> MSKGTTCQKAIVNWEAANPGKNPSEAEEIKLIFQIPPIEKMDGPVLNTLTKCKKLSLSSNSIDKMISLNMLRNLEILSLSRNVIKKISGLEDIGGTLRQLWLSYNFIEKLDGLNNCSVLQTLYIGNNRIKNWEELDKLKDLPELENVLFYGNPI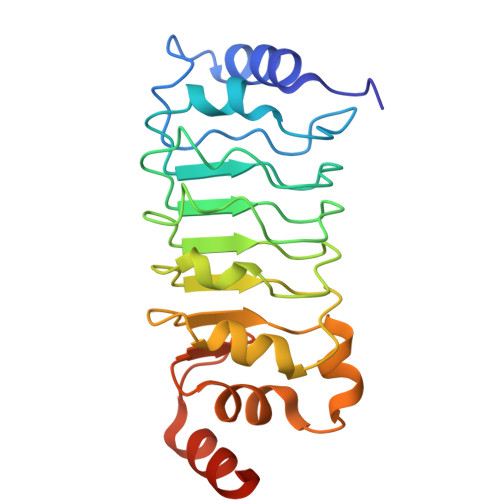YEQVKEDPKLIVLKKLPTLKNVDGYIIDDSVLEKVKQIADIPISAKQL> XSFAGLKDADVAAALAACSAADSFKHKEFFAKVGLASKSLDDVKKAFYVIDQDKSGFI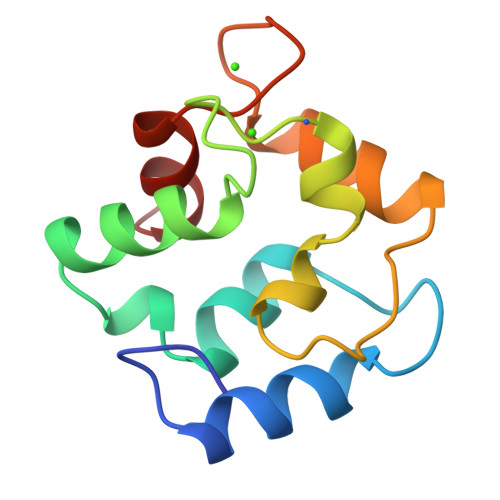EEDELKLFLQNFSPSARALTDAETKAFLADGDKDGDGMIGVDEFAAMIKA>AVVKDFDISKFLGFWYEIAFASKMGTPGLAHKEEKMGAMVVELKENLLALTTTYYSEDHCVLEKVTATEGDGPAKFQVTRLSGKKEVVVEATDYLTYAIIDITSLVAGAVHRTMKLYSRSLDDNGEALYNFRKITSDHGFSETDLYILKH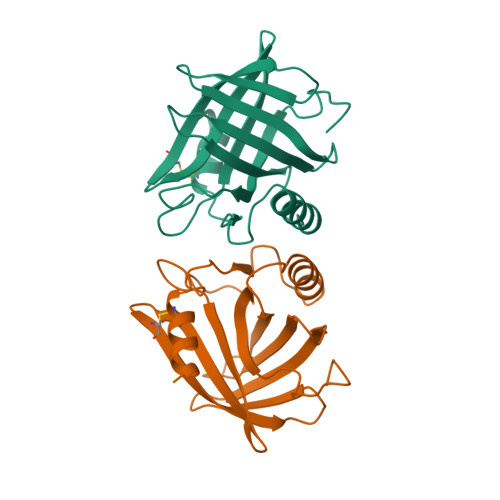DLTCVKVLQSAAES[2x]> GSMG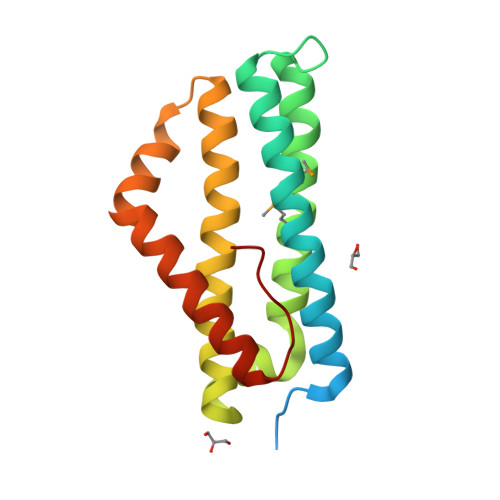EDEGEQTKTKKDSNKVVKTASRPKLSTKDLALIKADLAEFEARELSSEKILKDTIKEESWSDLDFANDNINQMIGTMKRYQQEILSIDAIKRASEASADTEAFKKIFKEWSEFKIERIQVTIDLLNGKKDSEAVFKKTYPNQIIFKKVRTNKLQTALNNLKVGYELLDSQK> MWSHPQFEKNQLQQLQNPGESPPVHPFVAPLSYLLGTWRGQGEGEYPTIPSFRYGEEIRFSHSGKPVIAYTQKTWKLESGAPALAESGYFRPRPDGSIEVVIACSTGLVEVQKGTYNVDEQSIKLKSDLVGNASKVKEISREFELVDGKLSYVVR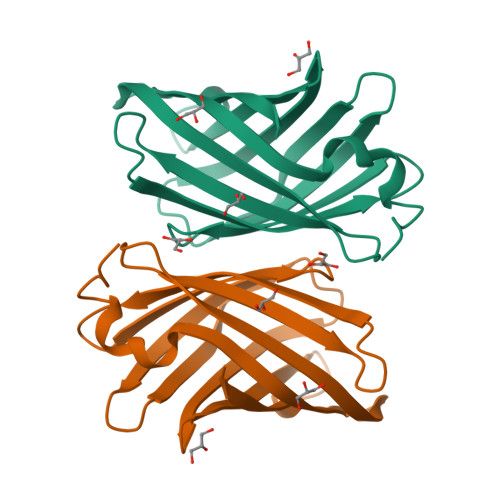LSTTTNPLQPALKAILDKL>[2x]GPTEGEAGELRIAVECHTCFDWLMPAMGEFRPMWPQVELDIVSGFQADPVGLLLQHRADLAIVSEAEKQNGISFQPLFAYEMVGICAPDHPLAAKNVWTAEDFIGETLITYPVPDEM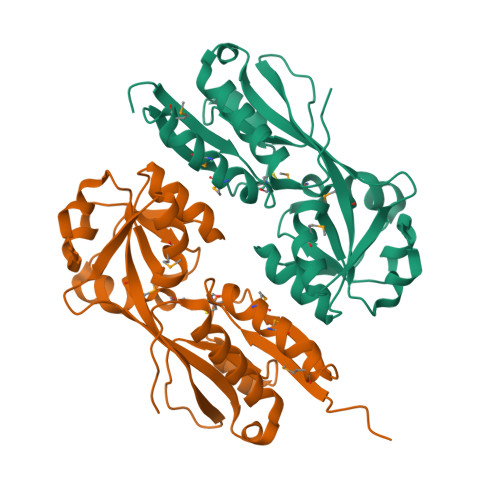LDLPKKILIPKNINPPRRHSELTIAIIQLVASRRGIAALPYWTVMPYLEKGYVVHRQITADGLQSKLYAAIRTEDTDKSYLNNFCQIIRERGFADLPGLSELEPV> ISGMSGRKASGSSPTSPINANKVENEDAFLEEVAEEKPHVKPYFTKTILDMEVVEGSAARFDCKVEGYPDPEVMWFKDDNPVKESRHFQIDYDEEGNCSLTISEVC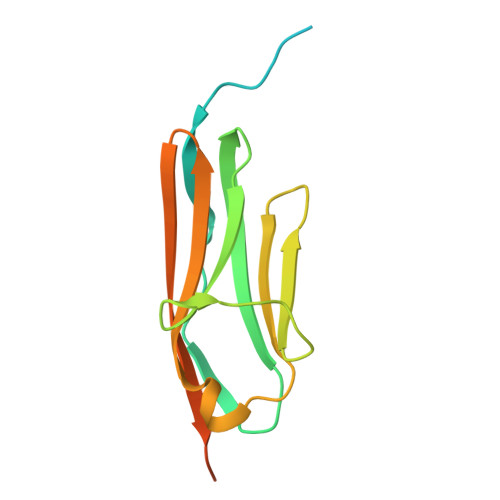GDDDAKYTCKAVNSLGEATCTAELLVETMGKEGEGEGEGEEDEEEEEE>MSGSHHHHHHSSGIEGRGRLIKHMTAEAGITG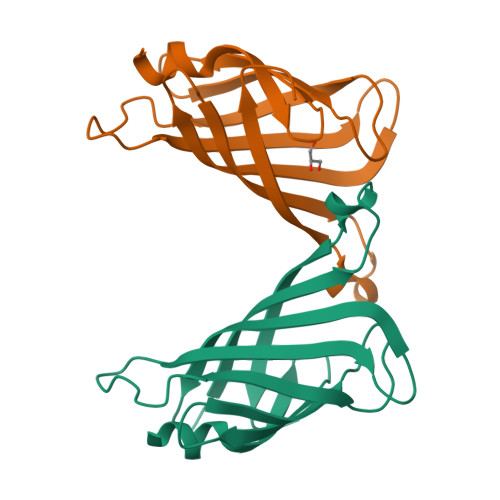TWYNQLGSTLIVTAGADGALTGTYESAVGNAEGSYVLTGRYDSAPATDGSGTALGWTVAWKNNYRNAHSASTWSGQYVGGAEARINTQVLTTSGTTEANAWKSTLVGHDTFTKVKPSAASI[2x]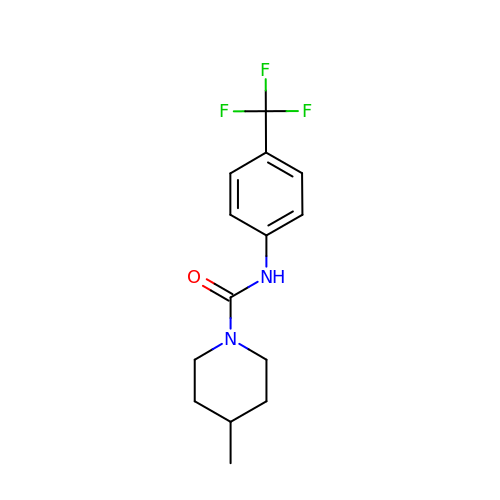4-methyl-~{N}-[4-(trifluoromethyl)phenyl]piperidine-1-carboxamide | C14 H17 F3 N2 O | GSJUDFGKALFBQN-UHFFFAOYSA-N> MPLDPVIQQVLDQLNRMPAPDYKHLSAQQFRSQQSLFPPVKKEPVAEVREFDMDLPGRTLKVRMYRPEGVEPPYPALVYYHGGGWVVGDLETHDPVCRVLAKDGRAVVFSVDYRLAPEHKFPAAVEDAYDALQWIAERAADFHLDPARIAVGGDSAGGNLAAVTSILAKERGGPA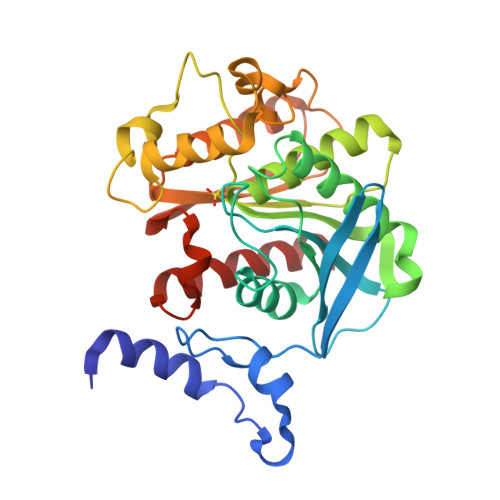LAFQLLIYPSTGYDPAHPPASIEENAEGYLLTGGMSLWFLDQYLNSLEELTHPWFSPVLYPDLSGLPPAYIATAQYDPLRDVGKLYAEALNKAGVKVEIENFEDLIHGFAQFYSLSPGATKALVRIAEKLRDALA> MSDLIEYSFYLTYAFLMTTGTITFIEALRTKNESVRHILNLETCISVVAAFFYSNFIGKLEHINYEEINLNRYVDWAITTPIMLLVLVLAFRVNQTNKAMVKFSDFMIIL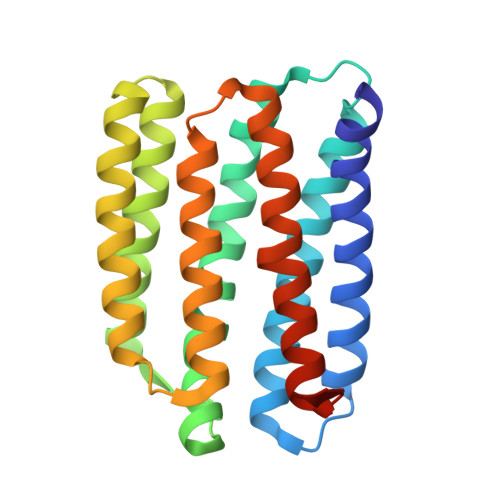GMNYGMLGTGYLGDIGVIHKTMGTVLGFLFFGGLFYKLNTLRTSNASNDLLYGAFFVLWALYGVFYQMEQLPRNVGYNVLDLFSKCFVGIYFWAFYAKIFTLEHHHHHH> GAMGSRKS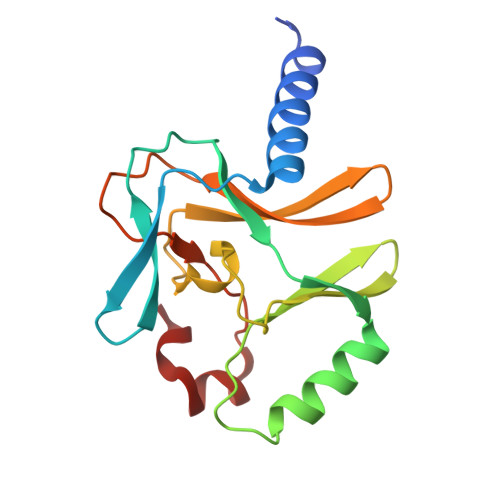KAELQSEERKRIDELIESGKEEGMKIDLIDGKGRGVIATKQFSRGDFVVEYHGDLIEITDAKKREALYAQDPSTGCYMYYFQYLSKTYCVDATRETNRLGRLINHSKCGNCQTKLHDIDGVPHLILIASRDIAAGEELLFDYGDRSKASIEAHPWLKH>[2x]MLEADDQGCIEEQGVEDSANEDSVDAKPDRSSFVPSLFSKKKKNVTMRSIKTTRDRVPTYQYNMNFEKLGKCIIINNKNFDKVTGMGVRNGTDKDAEALFKCFRSLGFDV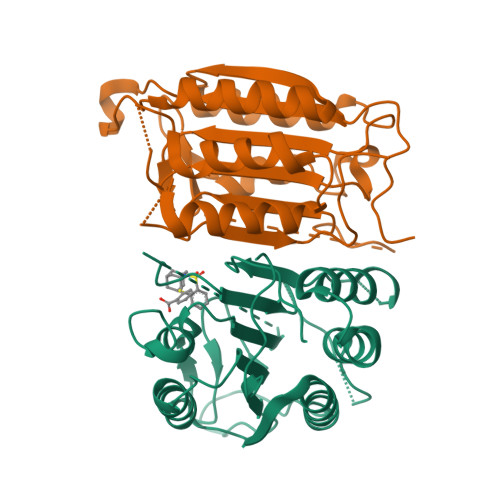IVYNDCSCAKMQDLLKKASEEDHTNAACFACILLSHGEENVIYGKDGVTPIKDLTAHFRGDRCKTLLEKPKLFFIQACRGTELDDGIQADSGPINDTDANPRYKIPVEADFLFAYSTVPGYYSWRSPGRGSWFVQALCSILEEHGKDLEIMQILTRVNDRVARHFESQSDDPHFHEKKQIPCVVSMLTKELYFSQ> APQAPASATPAKVPVIEWGKCEQLKPSESERTSKAAVVDKCLQSLPLPDPEKATQQEIDKHRESVTTCALKAEGWFDDEGVYKFDRARNEIKNKK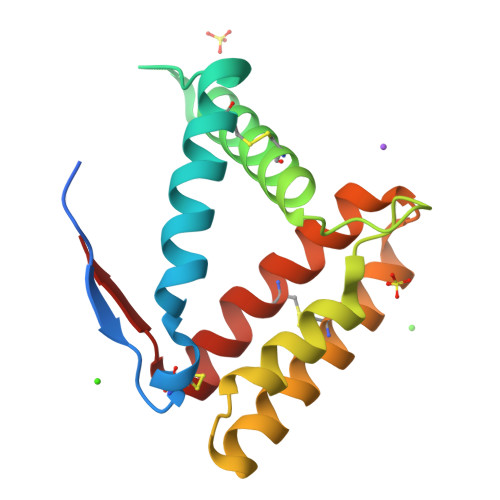LDSEVEEAVLLKHDACQKEATEKHDDYINQVQLYQACMDYNISQICGIKVMV>[6x]GANAMAHMGKTLRFEIVSGVNKGYFHTNSQSESLDLVGGIWQKIAKEEFEKSNIYVSAVIKPSKTVYNQEWGCPENGQETVVLTGVANEEFVDDIE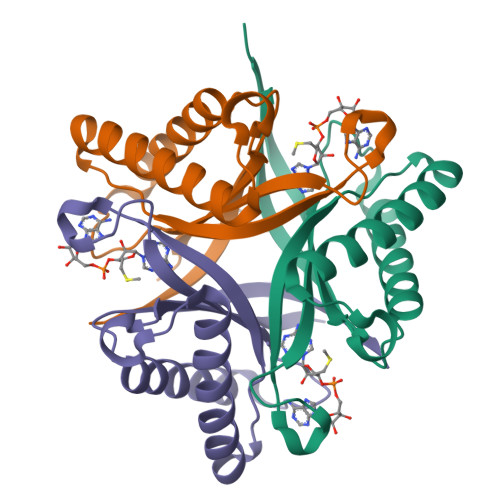KWKDTVIKLAKELKNQMKQSTLTCEFIETELHYFK>GPLGSVRDEIRSSVSDSVDEIVDGVSKT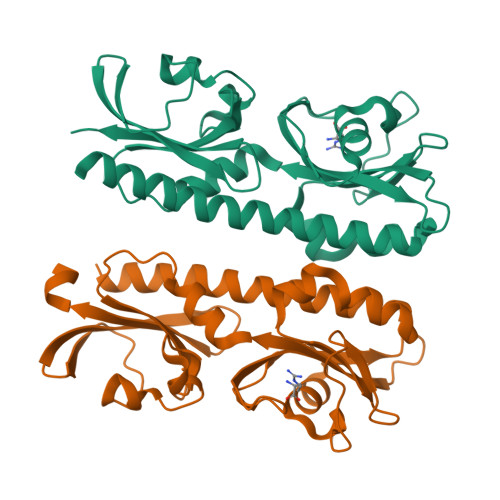TAEVINGRKSIAQYATSLIESNPEPDNVRTIISQPLIKNTFLLVGFGLEKDGSNINNDPSWNPGPTWDPRVRPWYKDAKNAGKLVITAPYADSASGEILVSVATPVKDSATGQFLGSIFYDVSLAELAELVNEVKLFDAGYVFIVSEDGTTIAHPKKEFNGKPMSEFLGESKINVDTHQVIINGKPYAVSFSDVEGEDWYVGVVIDEEIAYAALDELRRSTLIHHHHHH[2x]>[2x]MPKLVTWMNNQRVGELTKLANGAHTFKYAPEWLASRYARPLSLSLPLQRGNITSDAVFNFFDNLLPDSPIVRDRIVKRYHAKSRQPFDLLSEIGRDSVGAVTLIPEDETVTHPIMAWEKLTEARLEEVLTAYKADIPLGMIREENDFRISVAGAQEKTALLRIGNDWCIPKGITPTTHIIKLPIGEIRQPNATLDLSQSVDNEYYCLLLAKELGLNVPDAEIIKAGNVRALAVERFDRRWNAERTVLLRLPQEDMCQTFGLPSSVKYESDGGPGIARIMAFLMGSSEALKDRYDFMKFQVFQWLIGATDGHAKNFSVFI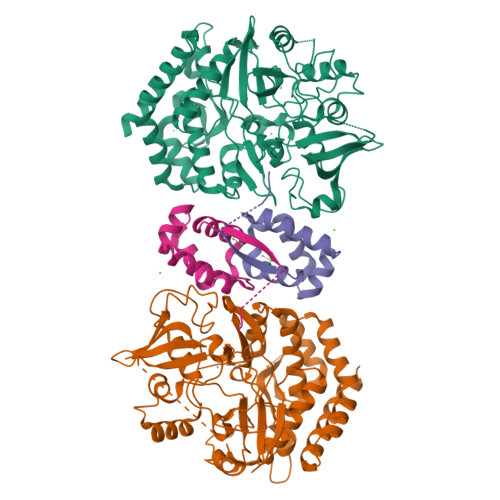QAGGSYRLTPFYDIISAFPVLGGTGIHISDLKLAMGLNASKGKKTAIDKIYPRHFLATAKVLRFPEVQMHEILSDFARMIPAALDNVKTSLPTDFPENVVTAVESNVLRLHGRLSREYGSKHHHHHH;>[2x]MMSFQKIYSPTQLANAMKLVRQQNGWTQSELAKKIGIKQATISNFENNPDNTTLTTFFKILQSLELSMTLCDAKNASPESTEQQNLEW> AERSELTIHPKEFTTFVRNFNPFLGATNLHTTTDFIYEPLVVFNEMHGNTPVFRLAENFQMSDDLMSVTFDIRKGVKWSDGEAFTADDVVYSFNLVKEKPELDQSGINSWVTGVEKVNDYQVKFRLSEANSNVPYEIAKVPVVPKHVWSKVKDPSTFTNENPVGSGPFTVIDTFTPQLYIQCEN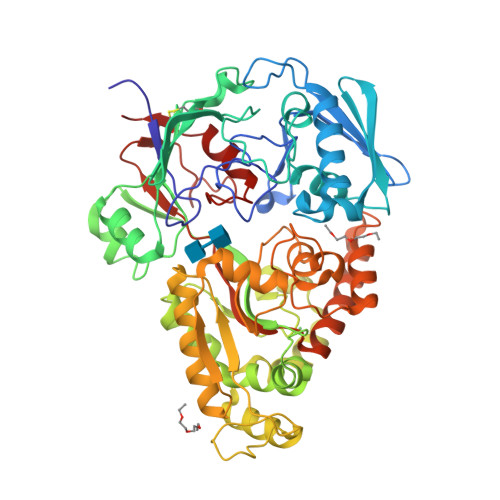PNYWDAANLDVDCLRVPQIANNDQFLGKVVNGEMDWTSSFVPDIDRTYAAASPKHHYWYPPAGTQAFVVNFKNPDAAKNEALTNVDFRRAFSMALDRQTIIDIAFYGGGTVNDFASGLGYAFEAWSDEKTHDKFKAYNSYNAEGAKKLLAKAGFKDVNKDGFVDTPSGKSFELLIQSPNGWTDFNNTVQLAVEQLAEVGIKARARTPDFSVYNQAMLEGTYDVAYTNYFHGADPYTYWNSAYNSALQSGDGMPRFAMHFYKNEKLDGLLNSFYKTADKQEQLEIAHGIQQIIAQDQVTIPVLSGAYMYQYNTTRFTGWWNEENPKGRPNIWAGIPERLLHVLDLKPVK The G-quadruplex and the i-motif are two noncanonical structures that have been studied extensively, and each is characterized by specific types of noncanonical interactions. G-quadruplexes (G4s) are formed from G-rich sequences and contain stacked guanosine tetrads, organized in a cyclic hydrogen bonding arrangement between the Hoogsteen and Watson–Crick faces of neighboring nucleobases. The DNA i-motif is characterized by the formation of hemiprotonated C–C+ parallel-stranded base pairs, which are organized to allow two duplexes to intercalate in an antiparallel fashion to form a quadruplex structure. As part of a screen to probe the structural diversity of DNA, we have crystallized many short DNA oligonucleotides, including d(CCAGGCTGCAA).

Initial phases from this derivative were used to create electron density maps for the higher resolution native structure. Refined native and derivative structures were virtually identical, with an RMSD of 0.377 Å for all DNA atoms of the asymmetric unit. Two distinct strands form a dimer through parallel-stranded interactions, while a symmetry-related dimer interacts in an antiparallel orientation to form the tetramer. The tetramer contains two central G-tetrads that are stabilized by a barium ion and are flanked on either side by a base triple, one unpaired guanosine and an i-motif of three C–C+ base pairs. The eight guanosines coordinate directly with a central cation that is located between the two G-tetrad planes. Both the native and U7-Br oligonucleotides were crystallized in the presence of barium chloride, and a strong (11 σ) anomalous difference electron density peak between the two G-tetrads was observed in both native and derivative structures. The Ba2+ ion lies on or very near a crystallographic symmetry axis with a refined final occupancy of 0.50 and B-factors of 73.27 Å2. The coordination distances between the cation and guanosine O6 positions range from 2.5 to 2.8 Å, with an average distance of 2.63 Å.

>[2x]CCAGGCUGCAA> MGSSHHHHHHENLYFQSNAMFSAGHKIKGTVVLMPKNELEVNPDGSAVDNLNAFLGRSVSLQLISATKADAHGKGKVGKDTFLEGINTSLPTLGAGESAFNIHFEWDGSMGIPGAFYIKNYMQVEFFLKSLTLEAISNQGTIRFVCNSWVYNTKLYKSVRIFFANHTYVPSETPAPLVEYREEELKSLRGNGTGERKEYDRIYDYDVYNDLGNPDKSEKLARPVLGGSSTFPYPRRGRTGRGPTVTDPNTEKQGEVFYVPRDENLGHLKSKDALEIGTKSLSQIVQPAFESAFDLKSTPIEFHSFQDVHDLYEGGIKLPRDVISTIIPLPVIKELYRTDGQHILKFPQPHVVQVSQ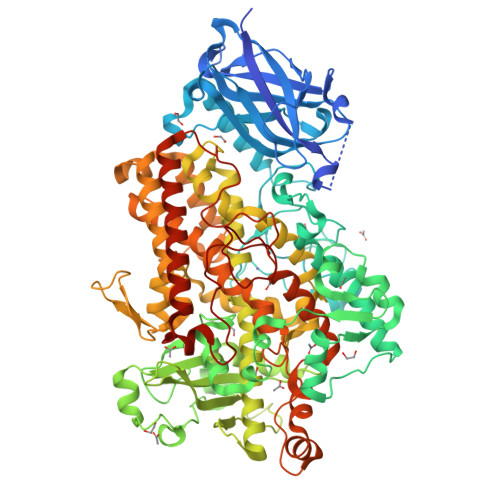SAWMTDEEFAREMIAGVNPCVIRGLEEFPPKSNLDPAIYGDQSSKITADSLDLDGYTMDEALGSRRLFMLDYHDIFMPYVRQINQLNSAKTYATRTILFLREDGTLKPVAIELSLPHSAGDLSAAVSQVVLPAKEGVESTIWLLAKAYVIVNDSCYHQLMSHWLNTHAAMEPFVIATHRHLSVLHPIYKLLTPHYRNNMNINALARQSLINANGIIETTFLPSKYSVEMSSAVYKNWVFTDQALPADLIKRGVAIKDPSTPHGVRLLIEDYPYAADGLEIWAAIKTWVQEYVPLYYARDDDVKNDSELQHWWKEAVEKGHGDLKDKPWWPKLQTLEDLVEVCLIIIWIASALHAAVNFGQYPYGGLIMNRPTASRRLLPEKGTPEYEEMINNHEKAYLRTITSKLPTLISLSVIEILSTHASDEVYLGQRDNPHWTSDSKALQAFQKFGNKLKEIEEKLVRRNNDPSLQGNRLGPVQLPYTLLYPSSEEGLTFRGIPNSISI2-(TOLUENE-4-SULFONYL)-2H-BENZO[D][1,2,3]DIAZABORININ-1-OL | 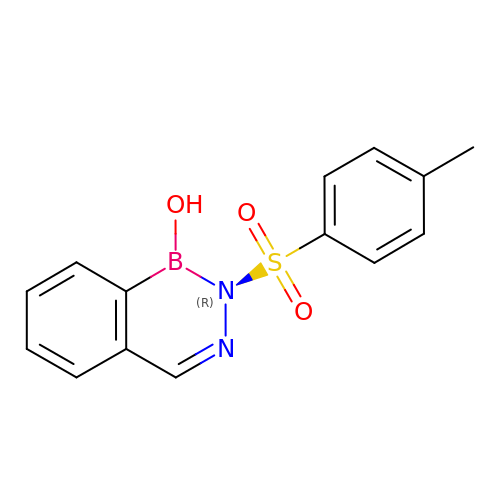C14 H13 B N2 O3 S | UQIDNSKBUXCODH-UHFFFAOYSA-N>M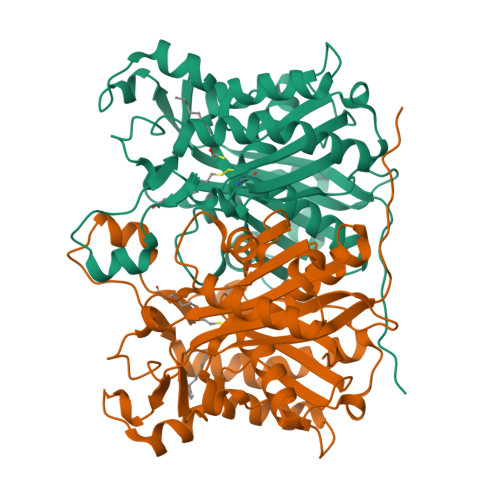TEIATTSGARSVGLLSVGAYRPERVVTNDEICQHIDSSDEWIYTRTGIKTRRFAADDESAASMATEACRRALSNAGLSAADIDGVIVTTNTHFLQTPPAAPMVAASLGAKGILGFDLSAGCAGFGYALGAAADMIRGGGAATMLVVGTEKLSPTIDMYDRGNCFIFADGAAAVVVGETPFQGIGPTVAGSDGEQADAIRQDIDWITFAQNPSGPRPFVRLEGPAVFRWAAFKMGDVGRRAMDAAGVRPDQIDVFVPHQANSRINELLVKNLQLRPDAVVANDIEHTGNTSAASIPLAMAELLTTGAAKPGDLALLIGYGAGLSYAAQVVRMPKG[2x]> MSLQGIHLSDLSYKHAILKESQYTIKRDVGTTTAVTPSSLQQEITLLCGEILYAKHADYKYAAEIGIQYISTALGSERVQQILRNSGSEVQVVLTRTYSLGKIKNNKGEDLQMLDIHGVEKSWVEEIDKEARKTMATLLKESSGNIPQNQRPSAPDTPIILLCVGALIFTKLASTIEVGLETTVRRANRVLSDALKRYPRMDIPKIARSFYDLFEQKVYHRSLFIEYGKALGSSSTGSKAESLFVNIFMQAYGAGQTMLRWGVIARSSNNIMLGHVSVQAELKQVTEVYDLVREMGPESGLLHLRQSPKAGLLSLANCPNFASVVLGNASGLGIIGMYRGRVPNTELFSAAESYAKSLKESNKINFSSLGLTDEEKEAAEHFLNVSDDSQNDYE

The viral genome is encapsidated in a sheath of oligomerized copies of the nucleoprotein N, forming a ribonucleoprotein complex termed nucleocapsid. The nucleocapsid is the template for transcription and replication by L, which is also dependent on the obligate polymerase cofactor, the phosphoprotein P, together forming the active L/P holoenzyme. In oligomerized and RNA-bound N (N-RNA) the nucleic acid is threaded along an extended groove in between the NTDs and CTDs of laterally connected N protomers. An important function of the C-terminal domain of P in nsNSVs is to bind to assembled N-RNA, forming an N-RNA/P complex.

Upon recombinant expression, N is known to take up host RNA and self-assemble into oligomers. Template-free 2D-classification of particles revealed that the sample contains primarily rings with 10 protomers. We obtained a 3.1 Å resolution map of 10-mer rings of N-RNA, a significant improvement from the previously reported crystallographic 10-mer at 4.2 Å33. We observed that the overall map quality was slightly better in the CTD region of N than in the NTD region, hinting at a degree of conformational heterogeneity in the NTD. we also determined a map of the 11-mer ring at 3.3 Å resolution. A structural alignment of the refined N protomer models solved by cryo-EM and crystallography shows that these are highly similar (r.m.s.d. of 0.5 Å). The 11-mer of N-RNA possesses a diameter of ~188 Å, slightly larger than the 10-mer at ~180 Å. The ring expansion by one protomer is accompanied by a slightly increased angle between neighboring N copies in the 11-mer: 73.6° in the 11-mer vs 72.0° in the 10-mer, in respect to the center of the rings. Thresholding of the map at a low level indicates the presence of additional N protomers, however, this density was too diffuse to fit more copies of N, presumably due to heterogeneity of the sample or conformational heterogeneity. It is notable that in this arrangement the RNA strand is obscured by N protomers belonging to the next turn of the assembly, suggesting that a conformational change is necessary for the genome to become accessible to L/P. Taking together our cryo-EM reconstructions, we observe that the lateral interaction of RNA-bound N protomers can support a range of geometries, demonstrating the plasticity of N-RNA and supporting the notion of a highly flexible HMPV nucleocapsid.>GPMPGKKVVARVAEAYAEDVGKRVVRVDKYERAKVGVKVGDYVEVKKV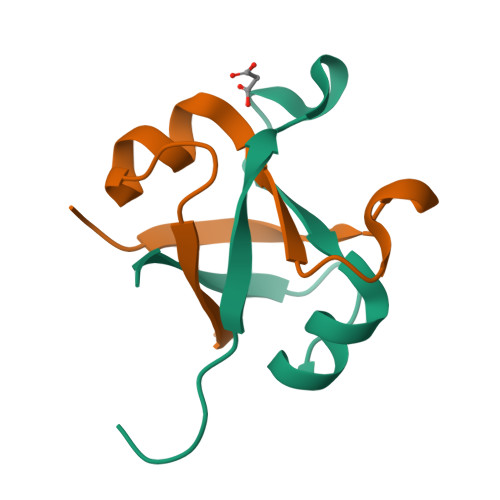[2x]> MRLLNRHSFVVKRKVSEDGYYNDDGDWVASQDIVEVNCKGNIQPYIKGSVKNGTQIALPEGIRLTDTRILY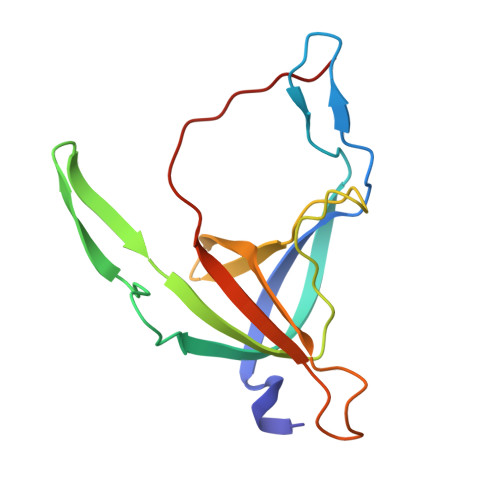TTYKLRTSDDVEWNESDIVMIDGHEYEVFMTMDWSQQLAHTSHYEYIIIRRDKMNAVRNSRT> GPKGPKGPKGKPGPEGEPGEPGEPGPKGPKG;> GPDGDPGDPGDPGP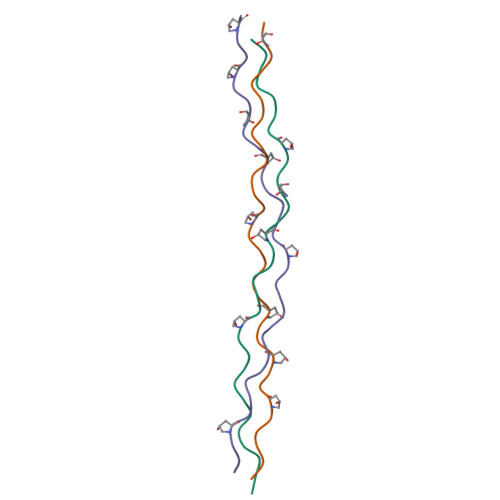DGRPGPDGPDGPAGDPG;> YGKPGPDGPDGPKGKPGPKGKPGKPGKPGKPG> GATIARTIVLQESIGKGRFGEVWRGKWRGEEVAVKIFSSREERSWFREAEIYQTVMLRHENILGFIAADNKDNGTWTQLWLVSDYHEHGSLFDYLNRYTVTVEGMIKLALSTASGLAHLHMEIVGTQGKPAIAHRDLKSKNILVKKNGTCCIADLGLAVRHDSATDTIDIAPNHRVGTKRYMAPEVLDDSINMKHFESFKRADIYAMGLVFWEIARRCSIGGIHEDYQLPYYDLVPSDPSVEEMRKVVCEQKLRPNIPNRWQSCEALRVMAKIMRE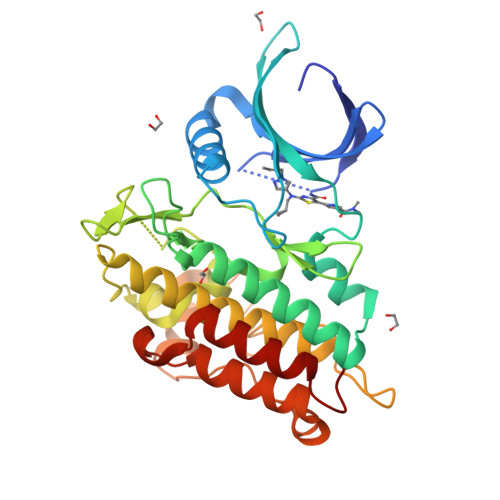CWYANGAARLTALRIKKTLSQLSQQEGIKM>[2x]MKESRAKKFQRQHMDSDSSPSSSSTYCNLMMLLRNMTQGRCKPVNTFVHEPLVDVQNVCFQEKVTCKNGQ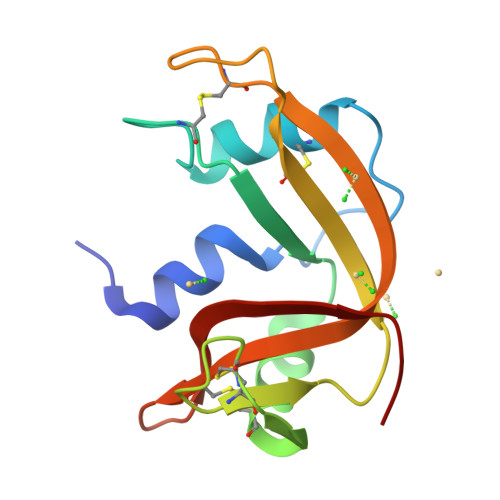GNCYKSNSSMHITDCRLTNGSRYPNCAYRTSPKERHIIVACEGSPYVPVHFDASVEDST(3E,5R)-8-(2-CHLOROPHENYL)-5-METHYL-2,6-DIOXOOCT-3-ENOATE | C15 H14 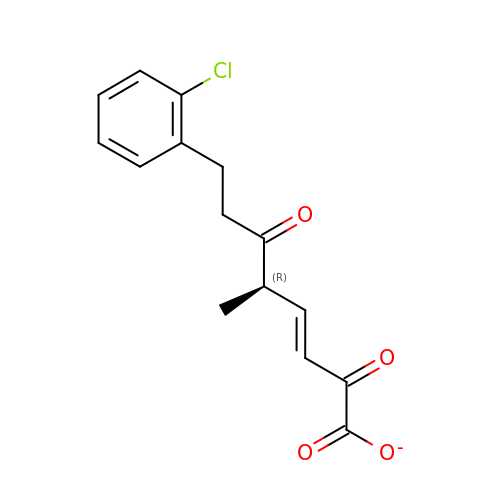Cl O4 | OXPYJYFFTOKNRF-QEHWCHDUSA-M>[2x]GSHMADGLTRREHDILAFERQWWKFAGVKEEAIKELFSMSATRYYQV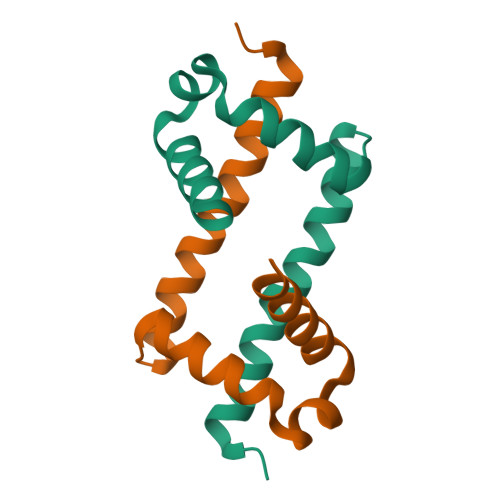LNALVDRPEALAADPMLVKRLRRLRASRQKA>[2x]MDIGINSDPPPRDWQLEKVVELSRHGIRPPTAGNREAIEAATGRPWTEWTTHDGELTGHGYAAVVNKGREEGQHYRQLGLLQAGCPTAESIYVRASPLQRTRATAQAL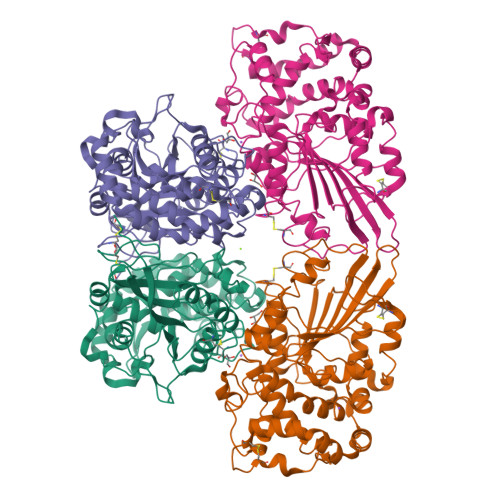VDGAFPGCGVAIHYANGDADPLFQTDKFAATQTDPARQLAAVKEKAGDLAQRRQALAPTIQLLKQAVCQADKPCPIFDTPWRVEQSKSGKTTISGLSVMANMVETLRLGWSENLPLSQLAWGKIAQASQITALLPLLTENYDLSNDVLYTAQKRGSVLLNAMLDGVKPEASPNVRWLLLVAHDTNIAMVRTLMNFSWQLPGYSRGNIPPGSSLVLERWRDAKSGERYLRVYFQAQGLDDLRRLQTPDAQHPMLRQEWRQPGCRQTDVGTLCPFQAAITALGQRIDRPSAPAVAMVLPKLAAALEHHHHHH6-(OCTAHYDRO-1H-INDOL-1-YLMETHYL)DECAHYDROQUINAZOLINE-2,4-DIAMINE | C17 H33 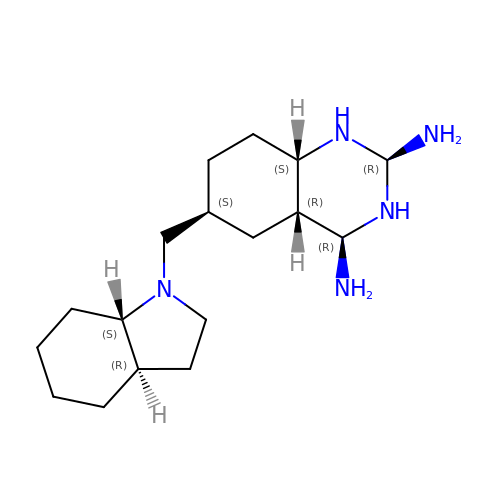N5 | HDQIGGQUKAQTGU-SZTTVXCBSA-N> MVPISPIETVPVKLKPGMDGPKVKQWPLTEEKIKALVEICTEMEKEGKISKIGPENPYNTPVFAIKKKDSTKWRKLVDFRELNKRTQDFWEVQLGIPHPAGLKKKKSVTVLDVGDAYFSVPLDEDFRKYTAFTIPSINNETPGIRYQYNVLPQGWKGSPAIFQSSMTKILEPFKKQNPDIVIYQYMDDLYVGSDLEIGQHRTKIEELRQHLLRWGLTTPDKKHQKEPPFLWMGYELHPDKWTVQPIVLPEKDSWTVNDICKLVGKLNWASQIYPGIKVRQLSKLLRGTKALTEVIPLTEEAELELAENREILKEPVHGVYYDPSKDLIAEIQKQGQGQWTYQIYQEPFKNLKTGKYARMRGAHTNDVKQLTEAVQKITTESIVIWGKTPKFKLPIQKETWETWWTEYWQATWIPEWEFVNTPPLVKLWYQLEKEPIVGAETFYVDGAANRETKLGKAGYVTNKG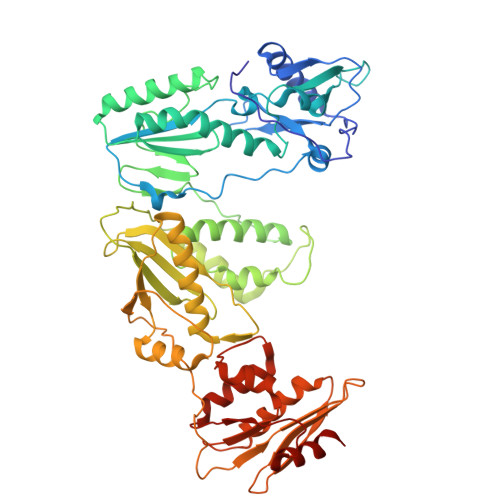RQKVVPLTNTTNQKTELQAIYLALQDSGLEVNIVTDSQYALGIIQAQPDKSESELVNQIIEQLIKKEKVYLAWVPAHKGIGGNEQVDKLVSAG>[4x]MGSAFYK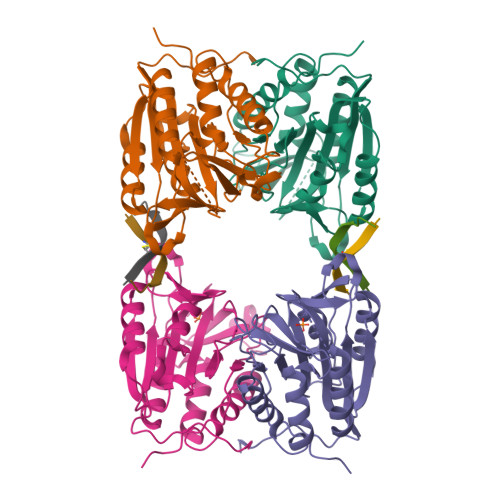REMFDPAEKYKMDHRRRGIALIFNHERFFWHLTLPERRGTCADRDNLTRRFSDLGFEVKCFNDLKAEELLLKIHEVSTVSHADADCFVCVFLSHGEGNHIYAYDAKIEIQTLTGLFKGDKCHSLVGKPKIFIIQAARGNQHDVPVIPLDVVDNQTEKLDTNITEVDAASVYTLPAGADFLMCYSVAEGYYSHRETVNGSWYIQDLCEMLGKYGSSLEFTELLTLVNRKVSQRRVDFCKDPSAIGKKQVPCFASMLTKKLHFFPKSNHHHHHH;>[4x]TEKEKGRLHCVEWTILER> G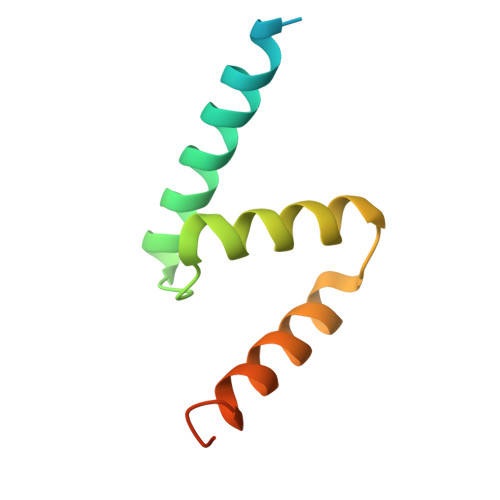PHMASSGGAGAAAAAAAANLNAVRETMDVLLEISRILNTGLDMETLSICVRLCEQGINPEALSSVIKELRKATEALKAAENMTS>[2x]TTK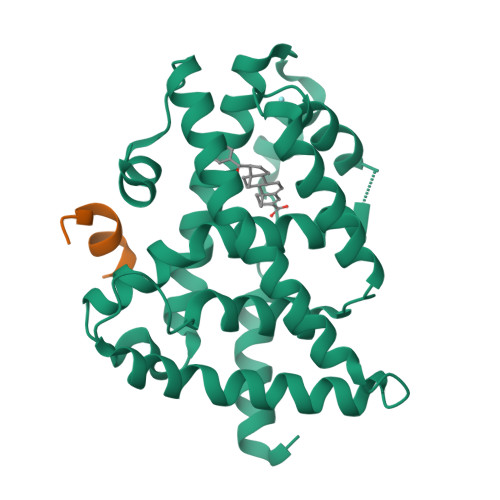SCREKTELTPDQQTLLHFIMDSYNKQRMPQEITNKILKEEFSAEENFLILTEMATNHVQVLVEFTKKLPGFQTLDHEDQIALLKGSAVEAMFLRSAEIFNKKLPSGHSDLLEERIRNSGISDEYITPMFSFYKSIGELKMTQEEYALLTAIVILSPDRQYIKDREAVEKLQEPLLDVLQKLCKIHQPENPQHFACLLGRLTELRTFNHHHAEMLMSWRVNDHKFTPLLCEIWDVQ;>[2x]CPSSHSSLTERHKILHRLLQEGSPS> GGUCCGUCCGGGUCCGUGGUUGCGUCGUUCAGGCGCCCGGUCUCCGGGUGCGCGAGCGACUAGCCGAUGCCAGUCGCAGGCAAAGCGGUCCACGUAACC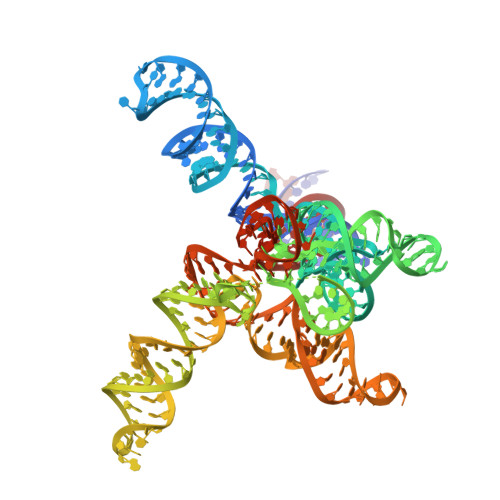CCGGCAACGGGGGAUCACGGUGCGGCUUAGACGUAAGUCCUGCCUCGUGGCCAUCGUCAGAUACGACGGCGUACGGGAGAAGGCCGGUAGUGGCAGAGAAGCUGCGGAAGCCUCAGCAGGCGAUUGUGGGGUCGAAGACCAGGUCGGCCGGACGGA Recently, a new Class 2 family of CRISPR nucleases named Cas12j, also known as CasΦ, was found in the biggiephage clade of phages. In addition, the RuvC catalytic site of Cas12j1 and 2 also processes the precursor crRNA (pre-crRNA). This family of endonucleases recognise protospacers with a minimal T-rich PAM, and their small size (700–800 residues) together with the lack of a transactivation crRNA (trac-crRNA) to build the functional RNP, make Cas12j an atypical family of miniaturized RNA-guided nucleases. Cas12j proteins share low sequence identity with other CRISPR nucleases and display sequence homology only in their RuvC domain with Class2 type V members. They generate a staggered DNA double-strand break (DSB) and unleash unspecific ssDNA cleavage after activation with an ssDNA complementary to the crRNA, as other members of Class 2 type V7,8.

We reconstituted a functional Cas12j3−crRNA complex and determined the structure of the enzyme after severing a target dsDNA by cryo-EM. The predominant class yielded a map at a resolution of 2.7 Å, which was used to build the model of the Cas12j3/R-loop structure. The R-loop displays a T shape with the crRNA/DNA hybrid and the crRNA handle forming the horizontal and vertical bars, and the protein domains wrapping around the nucleic acids. The N-terminal region comprises the T-strand and NT-strand PAM interacting domains (TPID, NPID) and the RNA-handle binding domain (RBD), while the C-terminal consists of the catalytic RuvC and stop (STP) domains. The target DNA cleavage yields a triple strand R-loop with the T-strand hybridized to the crRNA, while the dissociated PAM NT-strand is directed towards the catalytic pocket. Our structure shows that PAM recognition in Cas12j3 is achieved by combining interactions in both strands by the TPID and NPID domains. An antiparallel β-sheet formed by β11 and β12 splits the Watson-Crick base coupling after the dG+17:C + 17 pair; thus, limiting the hybrid length to 17 nucleotides in agreement with cleavage experiments testing the efficiency of the spacer length. The RuvC insertion runs alongside the crRNA strand of the hybrid, making multiple contacts with its phosphate backbone from U + 9 to G + 13. Interestingly, two nucleotides, modelled as purines, were observed in the active site in complex with Ni2+ as a by-product of the phosphodiester hydrolysis. A second metal atom, modelled as Zn, is coordinated by 4 conserved cysteines, similarly to Cas12g and the dimeric Cas12f33.

> MEKEITELTKIRREFPNKKFSSTDMKKAGKLLKAEGPDAVRDFLNSCQEIIGDFKPPVKTNIVSISRPFEEWPVSMVGRAIQEYYFSLTKEELESVHPGTSSEDHKSFFNITGLSNYNYTSVQGLNLIFKNAKAIYDGTLVKANNKNKKLEKKFNEINHKRSLEGLPIITPDFEEPFDENGHLNNPPGINRNIYGYQGCAAKVFVPSKHKMVSLPKEYEGYNRDPNLSLAGFRNRLEIPEGEPGHVPWFQRMDIPEGQIGHVNKIQRFNFVHGKNSGKVKFSDKTGRVKRYHHSKYKDATKPYKFLEESKKVSALDSILAIITIGDDWVVFDIRGLYRNVFYRELAQKGLTAVQLLDLFTGDPVIDPKKGVVTFSYKEGVVPVFSQKIVPRFKSRDTLEKLTSQGPVALLSVDLGQNEPVAARVCSLKNINDKITLDNSCRISFLDDYKKQIKDYRDSLDELEIKIRLEAINSLETNQQVEIRDLDVFSADRAKANTVDMFDIDPNLISWDSMSDARVSTQISDLYLKNGGDESRVYFEINNKRIKRSDYNISQLVRPKLSDSTRKNLNDSIWKLKRTSEEYLKLSKRKLELSRAVVNYTIRQSKLLSGINDIVIILEDLDVKKKFNGRGIRDIGWDNFFSSRKENRWFIPAFHKAFSELSSNRGLCVIEVNPAWTSATCPDCGFCSKENRDGINFTCRKCGVSYHADIDVATLNIARVAVLGKPMSGPADRERLGDTKKPRVARSRKTMKRKDISNSTVEAMVTA(4aS,7aR)-octahydro-1H-cyclopenta[b]pyridine-6,6-diylbis(phosphonic 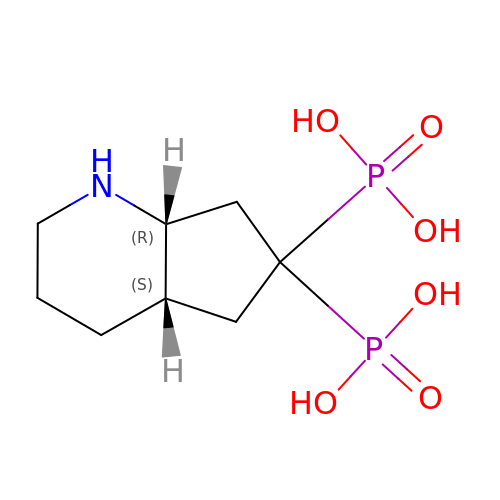acid) | C8 H17 N O6 P2 | JWOKHNWVYMHFTC-NKWVEPMBSA-N>[2x]MSAKDTADLSPLLEANRKWADECAAKDSTYFSKVAGSQAPEYLYIGCADSRVSPAQLFNMAPGEVFVQRNVGNLVSNKDLNCMSCLEYTVDHLKIKHILVCGHYNCGACKAGLVWHPKTAGVTNLWISDVREVRDKNAAKLHGLSADDAWDKMVELNVEAQVFNVCASPIVQAAWARGQPLSVHGIVYTPGTGLVKELIKPITGMEDAGALLRADLKQHCFFSESLA

Carbonic anhydrases (CAs, EC 4.2.1.1) are metalloenzymes, which catalyze the reversible hydration of carbon dioxide. In order to learn more about the molecular mechanism of β-CA, we have determined the crystal structure of β-CA from Coccomyxa (Co-CA) in complex with five inhibitors: acetazolamide, thiocyanate, azide, iodide, and phosphate ions. Co-CA is a homo-tetrameric structure with one dimer present in the asymmetric unit. The catalytic zinc ion binds to the side chains of residues Cys-47, His-103, and Cys-106 in a tetrahedral geometry with the fourth ligand expected to be a water molecule in the native enzyme.

Azide and thiocyanate ions in the active site of Co-CA were clearly defined in the 2.3 Å and 2.5 Å electron density maps, respectively. For SCN- the nitrogen atom is also positioned 2.0 Å from the zinc ion, and makes a comparable, but weaker, hydrogen bond to the amide group of Gly-107 (3.4 Å). The geometry of the zinc is tetrahedral — the four substituent atoms binding to the zinc ion in Co-CA-SCN have bond angles between 100° and 120°. There is a water molecule bridging the Asp-49 Oδ2 atom and the NH atom of Gly-107 in the SCN- inhibited structure. In Co-CA, thiocyanate binds tetrahedrally to the zinc ion analogous to acetazolamide, azide and water (this work and [17]). The orientation of the thiocyanate ion in the Mt-CA structure and in the Co-CA-SCN structure reported here is not identical. In Mt-CA, the sulphur atom of the inhibitor is positioned in the vicinity of Ala-75, i.e. the residue homologous to Val-71 in Co-CA. The sulphur atom in Co-CA-SCN is however directed towards Tyr-88′. For Co-CA-IOD and Co-CA-SCN, iodide and thiocyanate ions, respectively, substituted the chloride ions at the interface. The histidine side-chain has two conformations: an "in" conformation in Co-CA-SCN in which the side chain is directed towards the active site area, two conformations in Co-CA-AZM and Co-CA-PO4 (monomer B only, in monomer A it is "in"), and an "out" conformation in the structures of Co-CA-AZI, and Co-CA-IOD.> ETGQTLAANIWSDKTTAQNEPINLTNANAPIKNAKNLNSTITNVAAFDTKLNHLLVDTITGRVFVGGVNRLYQLSPDLELSETVKTGPQNDSVECSILDCPLNAVRSPTDNYNKVLLIDRATSRLIACGSLFQGTCTVRNLQNVSIIEHEVPDAVVANDANSSTVAFIAPGPPQHPVTNVMYVGVTYTNNSPYRSEIPAVASRSLEKTKMFQIASSAVTTGTRTFINSYARETYFVNYVYGFSSERFSYFLTTQLKHSHHSSPKEYITKLVRICQEDSNYYSYTEIPVECISDAQGGTKFNLVQAGFLGKPSSDLAQSLGISIQDDVLFAVFSKGEGNTPTNNSALCIYSLKSIRRKFMQNIKSCFNGSGMRGLDFISPSMPCVLTKLQTIGEDFCGLDVNSPLGGETPITSVPVAMFNTKLTSVAATSTSGYTVVFVGTSDGFLKKVVIESSSIANEYASFAVDLGSEINRDMQFDNQNLYIYVMSKTKVSKVKVFDCSDYKTCGDCLGARDPYCGWCSLENKCSPRSNCQDDANDPLYWVSYKTGKCTTITSVVPHQLQRTTARTLELIIDHLPQLKENLICAFTTEDKALFTNATKKRNGVNCTTPRTDMLPQIEQGKHHFTAKLSVRTRNGPDLVSTDFTFFDCSTHSSCTRCVSSEFPCDWCVEAHRCTHDTAENCRNDILVTGVSRIGPSYRSGPGFCPTGTKHHHHHH;> ETGDVKPDLQTKQDKVLAHFIGNSTDYFKILDHNDEFVLVGAKDVIYNVSLNGLKEIARLEWHSTDADRELCALKGKHEWDCHNYLRVYALRPNGEVLLCGTNSYKPRCRHYTPVEVSSEEAGSAGHAHAMRYEVSRDVEAQGLCPYSPAHNSTYAFADGHLYSATVADFSGGDPLIYRENLRTEQYDLKQLNQPDFVGAIERNGYVLFFFRELSMEVMNFGKAVYSRVARVCKNDRGGPYSHGKSWTSFLKARLNCSVPGEFPFYFDEIQAISPIVESGSKSLIYAVFTTSVNAIPGSAVCAFNVDDILAAFDGEFKSQKDSQSHWLPVEREQVPKPRPGQCVEDSRTLTSIAVNFIKNHPLMEEAVPAVHGRPLLTKVNLHHRLTAIAVHPQVKSLSGAYYDVIYSGTDDGKVTKFINILSTHPNSTVDRLKTVVISEMQVLPLGTPIRELVISTSKNSLVVVSDGSLVSVPLHHCSHIVDCLGCLSLQDPICAWDLQTHECKNLATSQHKFGTKTYLQSLNSTKKAAALLCPHIPRDAPGAETVSFVTMAPPPTEEQKLLYSNVGSGTKHHHHHH

Semaphorin ligands interact with plexin receptors to contribute to functions in the development of myriad tissues including neurite guidance and synaptic organisation within the nervous system. Cell‐attached semaphorins interact in trans with plexins on opposing cells, but also in cis on the same cell. We have discovered a distinct mode of interaction through which the Drosophila semaphorin Sema1b and mouse Sema6A mediate binding in cis to their cognate plexin receptors. Sema1a and Sema1b are most closely related to the mammalian class 6 semaphorins and interact with the sole Drosophila class A plexin, PlexA.

We next determined crystal structures of the PlexA1‐4‐Sema1b1‐2 complex from two different crystal forms (1:1 complex and 2:2 complex) at 3.0 and 4.8 Å resolution. The 1:1 complex crystal lattice contains one PlexA1‐4 monomer and one Sema1b1‐2 monomer per asymmetric unit. The crystal packing provides no Sema1b1‐2 dimerisation resembling that of the generic homodimeric architecture. The Sema1b1‐2 bound in the 1:1 complex with PlexA1‐4 is very similar to the unbound Sema1b1‐2 with the Cα rmsd of 0.81 Å indicating no large conformational changes upon complex formation. Only small differences in loop orientations at the ligand–receptor interface are apparent. The PlexA1‐4 structure in the 1:1 complex contains a sema domain composed of a seven‐bladed β‐propeller fold, which is followed by a PSI domain; however, we were not able to locate the IPT1‐PSI2 domain segment. The sema domain of PlexA is most similar to mouse PlxnA2 with an rmsd of 1.43 Å over 424 matched Cα positions. In the 1:1 complex crystal structure, PlexA1‐4 and Sema1b1‐2 interact through their sema domains in a head‐to‐head orientation similar to the generic architecture shared by all reported structures of semaphorin–plexin complexes (Janssen et al, 2010; Liu et al, 2010; Nogi et al, 2010). The PlexA1‐4‐Sema1b1‐2 interface buries a total solvent‐accessible area of 1,837 Å2. This extensive interface is composed of a mixture of hydrophobic and hydrophilic interactions similar to that of PlxnA2‐Sema6A.> VDEKYPSKYDNIDLDEILANKRLLTAYVNCIMERGKCSPEGKELKEHLVDAIETGCSKCTEAQEKGAYKVIEHLIQNELDTWHELT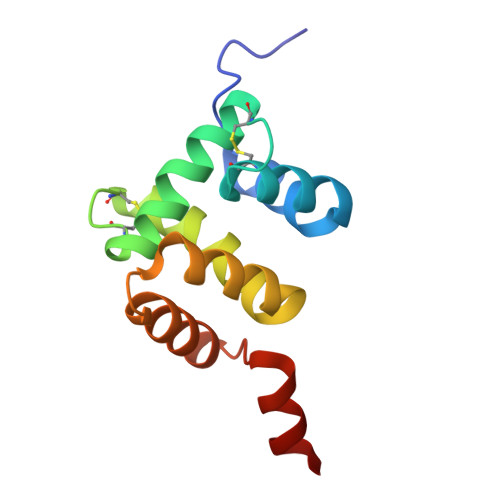DKYDSSGKWRKTYEDRARANGIVIPELEHHHHHH>MTTIRGDDLSNQITQISGSSSKKEEEKKKQQMLTGVLGLQPTMANHPVLGVFLPKYAKQNGGNVDKTAFRLDLIRMLALHRLNTKTGSD[16x];>MNSKSSARAAIVDTVEAVKKRKYISIEAGTLNNVVEKERKFLKQFLSGRENLRIAARVFTPCELLAPELENLGMLMYRFETDVDNPKILFVGLFFLCSNAFNVSACVRTALTTMYTNSMVDNVLSMINTCKYLEDKVSLFGVTSLVSCGSSCLLSCVMQGNVYDANKENIHGLTVLKEIFLEPDWEPRQHSTQYVYVVHVYKEVLSKLQYGIYVVLTSFQNEDLVVDILRQYFEKERFLFLNYLINSNTTLSYFGSVQRIGRCATEDIKSGFLQYRGITLPVIKLENIFVDLSEKKVFV[5x];>METVYCTFDHKLSLSDISTLCKLMNIVIPIPAHHHLIGSGNLGLYPIVSSNKDYVHIRNVLRTMVVTILQKVEGNQLVLRKPMTGQQYAIKNTGPFPWEKGDTLTLIPPLSTHSEEKLLKLGDWELTVPLVVPTAIAAEINIRLLCIGLIAVHREYNEMQTIIDELCSIQYRDVLIKLPDIVNDKQSMYSMKTACISLSMITAMAPDIVRTYIDRLTLEDHSMLLIKCQELLSKRTTLSTQRCGQLHATDIKDELKKIKSVLTMIDQINSLTNEKTYFVVCDVSADNRMATCIYKN[10x];>[16x]MENWQATEILPKIEAPLNIFNDIKTYTAEQLFDNLRIYFGDDPSRYNISFEALLGIYCNKIEWINFFTTPIAVAANVIRFNDVSRMTLGKVLFFIQLPRVATGNDVTAPKETTIMVAKHSEKHPINISFDLSAACLEHLENTFKNTVIDQILNINALHTVLRSLKNSADSLERGLIHAFMQTLLRKSPPQFIVLTMNENKVHNKQALSRVQRSNMFQSLKNRLLTSLFFLNRNNNSSYIYRILNDMMESVTESILNDTNNYTSKENIPLDGVLLGPIGSIQKLTNILSQYISTQVVSAPISYGHFIMGKENAVTAIAYRAIMADFTQFTVNAGTEQQDTNNKSEIFDKSRAYADLKLNTLKLGDKLVAFDHLHKVYKNTDVNDPLEQSLQLTFFFPLGIYIPTETGFSTMETRVKLNDTMENNLPTSVFFHNKDQVVQRIDFADILPSVCHPIVHDSTIVERLMKNEPLPTGHRFSQLCQLKITRENPTRILQTLYNLYESRQEVPKNTNVLKNELNVEDFYKPDNPTLPTERHPFFDLTYIQKNRATEVLCTPRIMIGNMPLPLAPISFHEARTNQMLEHAKTNSHNYDFTLKIVTESLTSGSYPELAYVIEILVHGNKHAFMILKQVISQCISYWFNMKHILLFCNSFEMIMLISNHMGDELIPGAAFAHYRNLVSLIRLVKRTISISNINEQLCGEPLVNFANALFDGRLFCPFVHTMPRNDTNAKITADDTPLTQNTVRVRNYEISDVQRMNLIDSSVVFTDNDRPSNENTILSKIFYFCVLPALSNNKACGAGVNVKELVLDLFYTEPFICPDDCFQENPISSDVLMSLIREAMGPGYTVANTSSIAKQLFKSLIYINENTKILEVEVSLDPAQRHGNSVHFQSLQHILYNGLCLISPITTLRRYYQPIPFHRFFSDPGICGTMNADIQVFLNTFPHYQRNDGGFPLPPPLALEFYNWQRTPFSVYSAFCPNSLLSIMTLAAMHSKLSPVAIAIQSKSKIHPGFAATLVRTDNFDVECLLYSSRAATSIILDDPTVTAEAKDIVTTYNFTQHLSFVDMGLGFSSTTATANLKRIKSDMGSKIQNLFSAFPIHAFTNTDINTWIRHHVGIEKPNPSEGEALNIITFGGINKNPPSILLHGQQAICEVILTPVTTNINFFKLPHNPRGRESCMMGTDPHNEEAARKALYDHTQTDSDTFAATTNPWASLPGSLGDILYNTAHREQLCYNPKTYSPNAQFFTESDILKTNKMMYKVINEYCMKSNSCLNSDSEIQYSCSEGTDSFVSRPCQFLQNALPLHCSSNQALLESRSKTGNTQISETHYCNYAIGETIPLQLIIESSI;>[12x]MDLKAQSIPFAWLDRDKVQRLTNFLSNLENLENVDLREHPYVTNSCVVREGEDVDELKTLYNTFILWLMYHYVLSKRKPDYNAIWQDITKLQNVVNEYLKSKGLNKGNFENMFTNKEKFESQFSDIHRALLRLGNSIRWGSNVPIDTPYVNLTAEDSSEIENNLQDAEKNMLWYTVYNINDPWDENGYLVTSINKLVYLGKLFVTLNQSWSKLEKVAMSQIVTTQNHLSGHLRKNENFNAVYSQRVLQTPLTGQRVESFLKIITSDYEIIKSSLESYSASKAFSVPENGPHSLMDFASLDGRMPSDLSLPSISIDTKRPSADLARLKISQPKSLDAPLKTQRRHKFPESDSVDNAGGKILIKKETLGGRDVRATTPVSSVSLMSGVEPLSSLTSTNLDLRDKSHGNYRIGPSGILDFGVKLPAEAQSNTGDVDLLQDKTSIRSPSSGITDVVNGLANLNLRQNKSDVSRPWSKNTAANADVFDPVHRLVSEQTGTPFVLNNSDVAGSEAKLTTHSTETGVSPHNVSLIKDLRDKDGFRKQKKLDLLGSWTKEKNDKAIVHSREVTGDSGDATETVTARDSPVLRKTKHANDIFAGLNKKYARDVSRGGKGNSRDLYSGGNAEKKETSGKFNVDKEMTQNEQEPLPNLMEAARNAGEEQYVQAGLGQRVNKILAEFTNLISLGEKGIQDILHNQSGTELKLPTENKLGRESEEANVERILEVSDPQNLFKNFKLQNDLDSVQSPFRLPNADLSRDLDSVS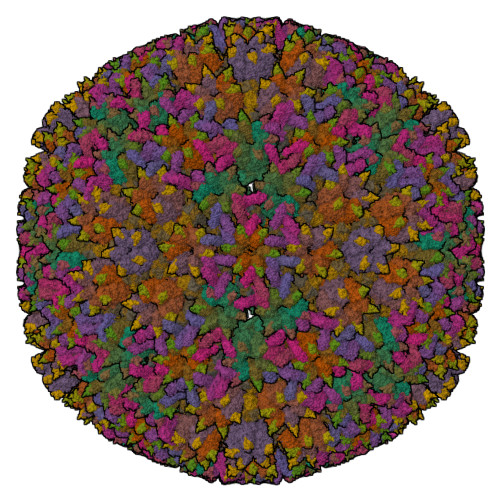FKDALDVKLPGNGEREIDLALQKVKAGERETSDFKVGQDETLIPTQLMKVETPEEKDDVIEKMVLRIRQDGETDEETVPGPGVAESLGIAAKDKSVIAS>GGCCCC[4x]

The abnormal expansion of GGGGCC/GGCCCC hexanucleotide repeats (HR) in C9orf72 is associated with amyotrophic lateral sclerosis (ALS) and frontotemporal dementia (FTD). On the RNA level, bidirectional transcription produces sense and antisense transcripts containing complementary regions of repeated stretches of GGGGCC (G4C2) and GGCCCC (G2C4) that form stable secondary and tertiary structures. Overall, the RNA folded into a parallel triplex-like motif flanked by double-stranded duplexes and terminated by single-stranded cytosines. The triplex motif was composed of four C+•G-C pairs representing standard major groove base triples (C+ denotes protonated cytosine).

ANP77 interacted with two neighboring single-stranded cytosines to form pseudo-canonical base pairs by adopting sandwich-like conformation and adjusting the position of its naphthyridine units to the helical twist of the RNA. In the G2C4–ANP77 structure, one ligand molecule was present. It interacted with the two overhanging cytosines of chain A, forming two pseudo-canonical base pairs. The NUs of ANP77 mimicked the nitrogen bases of nucleotides, forming three H-bonds with the functional groups of the overhanging cytosines from chain A at their Watson-Crick edges. The second pair of overhanging cytosines from chain D was ordered and interacted with symmetry-related RNA and the 2-exo amino group of the ligand. In the presented model, ANP77 exhibited a sandwich-like conformation, with the NUs shifting in relation to each other, resulting in limited stacking interactions between the aromatic moieties of the ligand. One of the NUs overlapped extensively with the neighbouring 1G from chain B, while the second unit did not form stacking interactions, despite its close proximity to the G–C pair of symmetry-related RNA molecules. The aminopropyl carboxamide side chain of ANP77 was located in the major groove of RNA. The crystallographic model of the G2C4-ANP77 complex confirmed that the ligand was capable of interacting directly with two consecutive cytosines. In the liganded structure three chloride ions were located: two in the major groove of the triplex motif and the third ion between the end of the triplex and beginning of the flanking duplex.>MAILDSAGVTTVTENGGGEFVDLDRLRRRKSRSDSSNGLLLSGSDNNSPSDDVGAPADVRDRIDSVVNDDAQGTANLAGDNNGGGDNNGGGRGGGEGRGNADATFTYRPSVPAHRRARESPLSSDAIFKQSHAGLFNLCVVVLIAVNSRLIIENLMKYGWLIRTDFWFSSRSLRDWPLFMCCISLSIFPLAAFTVEKLVLQKYISEPVVIFLHIIITMTEVLYPVYVTLRCDSAFLSGVTLMLLTCIVWLKLVSYAHTSYDIRSLANAADKANPEVSYYVSLKSLAYFMVAPTLCYQPSYPRSACIRKGWVARQFAKLVIFTGFMGFIIEQYINP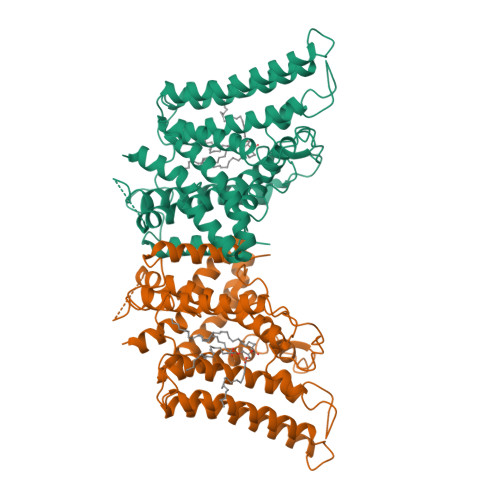IVRNSKHPLKGDLLYAIERVLKLSVPNLYVWLCMFYCFFHLWLNILAELLCFGDREFYKDWWNAKSVGDYWRMWNMPVHKWMVRHIYFPCLRSKIPKTLAIIIAFLVSAVFHELCIAVPCRLFKLWAFLGIMFQVPLVFITNYLQERFGSTVGNMIFWFIFCIFGQPMCVLLYYHDLMNRKGSMSGPHHHHHH[2x]>MKMASTRCKLARYLEDLEDVDLKKFKMHLEDYPPQKGCIPLPRGQTEKADHVDLATLMIDFNGEEKAWAMAVWIFAAINRRDLYEKAKRDEPKWGSDNARVSNPTVICQEDSIEEEWMGLLEYLSRISICKMKKDYRKKYRKYVRSRFQCIEDRNARLGESVSLNKRYTRLRLIKEHRSQQEREQELLAIGKTKTCESPVSPIKMELLFDPDDEHSEPVHTVVFQGAAGIGKTILARKMMLDWASGTLYQDRFDYLFYIHCREVSLVTQRSLGDLIMSCCPDPNPPIHKIVRKPSRILFLMDGFDELQGAFDEHIGPLCTDWQKAERGDILLSSLIRKKLLPEASLLITTRPVALEKLQHLLDHPRHVEILGFSEAKRKEYFFKYFSDEAQARAAFSLIQENEVLFTMCFIPLVCWIVCTGLKQQMESGKSLAQTSKTTTAVYVFFLSSLLQPRGGSQEHGLCAHLWGLCSLAADGIWNQKILFEESDLRNHGLQKADVSAFLRMNLFQKEVDCEKFYSFIHMTFQEFFAAMYYLLEEEKEGRTNVPGSRLKLPSRDVTVLLENYGKFEKGYLIFVVRFLFGLVNQERTSYLEKKLSCKISQQIRLELLKWIEVKAKAKKLQIQPSQLELFYCLYEMQEEDFVQRAMDYFPKIEINLSTRMDHMVSSFCIENCHRVESLSLGFLHNMPKEEEEEEKEGRHLDMV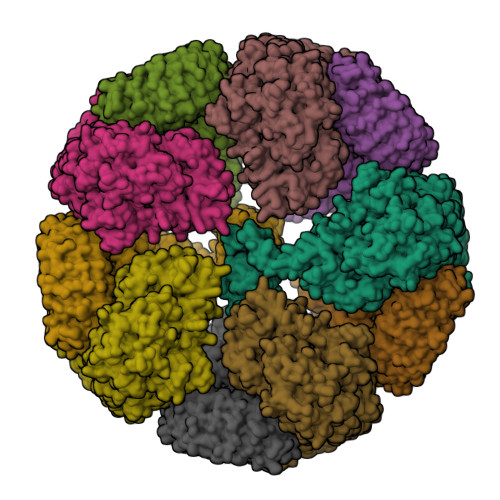QCVLPSSSHAACSHGLVNSHLTSSFCRGLFSVLSTSQSLTELDLSDNSLGDPGMRVLCETLQHPGCNIRRLWLGRCGLSHECCFDISLVLSSNQKLVELDLSDNALGDFGIRLLCVGLKHLLCNLKKLWLVSCCLTSACCQDLASVLSTSHSLTRLYVGENALGDSGVAILCEKAKNPQCNLQKLGLVNSGLTSVCCSALSSVLSTNQNLTHLYLRGNTLGDKGIKLLCEGLLHPDCKLQVLELDNCNLTSHCCWDLSTLLTSSQSLRKLSLGNNDLGDLGVMMFCEVLKQQSCLLQNLGLSEMYFNYETKSALETLQEEKPELTVVFEPSW[10x]> GGGKRYRAVYD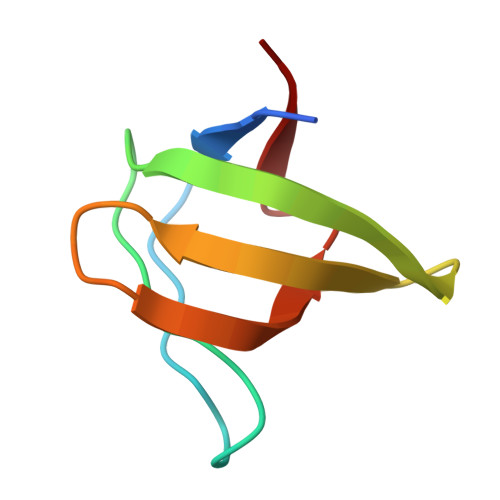YSAADEDEVSFQDGDTIVNVQQIDDGWMYGTVERTGDTGMLPANYVEAI Orthologous proteins to ependymin called ependymin-related proteins (EPDRs) have been found to exist in various tissues from sea urchins to humans, yet their functional role remains to be revealed. All of the EPDR1s fold into a dimer using a monomeric subunit that is mostly made up of two stacking antiparallel β-sheets with a curvature on one side, resulting in the formation of a deep hydrophobic pocket. All six of the cysteine residues in the monomeric subunit participate in the formation of three intramolecular disulfide bonds. The EPDR1 fold is very similar to the folds of bacterial VioE and LolA/LolB, which also use a similar hydrophobic pocket for their respective functions as a hydrophobic substrate-binding enzyme and a lipoprotein carrier, respectively.

A total of four monomeric subunits of EPDR1 were located in the asymmetric units of the human and mouse EPDR1 crystals. The refined structures showed average Cα r.m.s.d.s of 0.5 Å among the four human EPDR1 molecules and 1.0 Å among the four mouse EPDR1 molecules. BSAs of ∼2300 Å2 (per subunit) were calculated for these dimeric interfaces. Fish EPDR showed glycosylation at two asparagine sites, and the human, mouse and frog EPDR1s had two predicted N-glycosylation sites that were all conserved. Although glycosylation at these Asn residues in human and frog EPDR1 was only slightly perceivable and was too disordered to be modeled accurately as sugars, the glycosylation at the two Asn sites (Asn130 and Asn182) was well ordered in the case of mouse EPDR1 [Figs. 3(a) and 3(b)]. While the sugar modification at Asn130 could be modeled with only one N-acetylglucosamine (NAG), that at Asn182 was sufficiently ordered to be modeled with two NAGs (β-1,4 glycosidic bond) and one fucose attached to NAG (α-1,4 glycosidic bond). Such sugar modification is as expected for the initial glycosylation pattern in proteins expressed in insect cells. Interestingly, although Asp121, Pro122, Asp124 and Glu175 are conserved throughout the frog, mouse and human EPDR1s, a phenyl­alanine substitutes for Tyr177 of frog EPDR1 in both mouse and human EPDR1s. Since the hydroxyl group of Tyr177 stabilizes one of the water molecules that bind to the Ca2+ ion, it is expected that the mouse and human EPDR1s would be likely to have weaker binding to the metal.

>ADPHHHHHHHHTPQPCQAPQQWEGRQVLYQQSSGHNNRALVSYDGLNQRVRVLDERKALIPCKRLFEYILLYKEGVMFQIEQATKQCAKIPLVESWDPLDIPQNSTFEDQYSIGGPQEQILVQEWSDRRTARSYETWIGVYTAKDCYPVQETFIRNYTVVMSTRFFDVQLGIKDPSVFTPPSTCQAAQPEKMSDGCSL[4x]>NYEKLKNRLVQNARVAARQKEYTEIPDIFLCPISKTLIKTPVITAQGKVYDQEALSNFLIATGNKDETGKKLSMDDVVVFDELYQQIKVYNFYR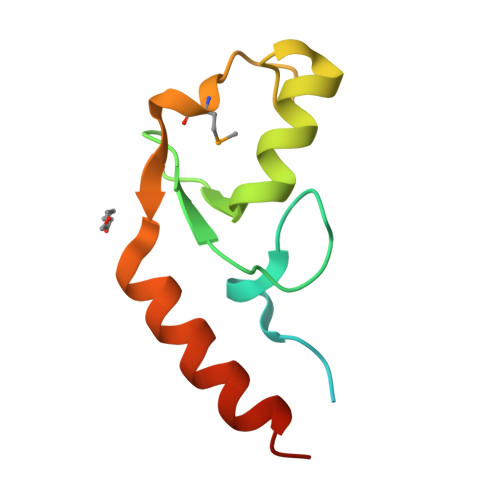KREVQKN[3x]> HHHHHHGLIQERRSHEVNPAAHLTGANSSLTGSGGPLLWETQLGLAFLRGLSYHDGALVVTKAGYYYIYSKVQLGGVGCPLGLASTITHGLYKRTPRYPEELELLVSQQSPCGR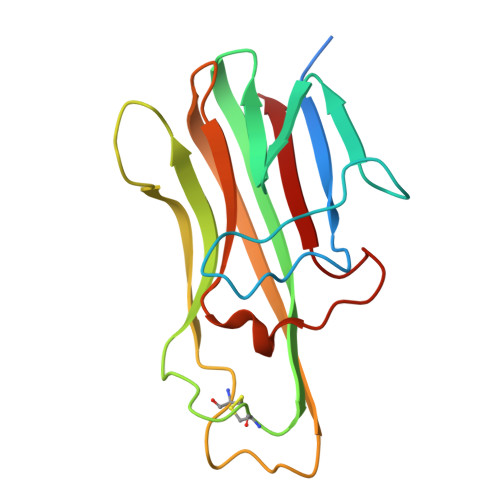ATSSSRVWWDSSFLGGVVHLEAGEEVVVRVLDERLVRLRDGTRSYFGAFMV>MNPAAEAEFNILLATDSYKVTHYKQYPPNTSKVYSYFECREKKTENSKLRKVKYEETVFYGLQYILNKYLKGKVVTKEKIQEAKDVYKEHFQDDVFNEKGWNYILEKYDGHLPIEIKAVPEGFVIPRGNVLFTVENTDPECYWLTNWIETILVQSWYPITVATNSREQKKILAKYLLETSGNLDGLEYKLHDFGYRGVSSQETAGIGASAHLVNFKVTDTVAGLALIKKYYGTKDPVPGYSVPAAEHSTITAWGKDHEKDAFEHIVTQFSSVPVSVVSDSYDIYNACEKIWGEDLRHLIVSRSTQAPLIIRPDSGNPLDTVLKVLEILGKKFPVTENSKGYKLLPPYLRVIQGDGVDINTLQEIVEGMKQKMWSIENIAFGSGGGLLQKLTRDLLNCSFKCSYVVTNGLGINVFKDPVADPNKRSKKGRLSLHRTPAG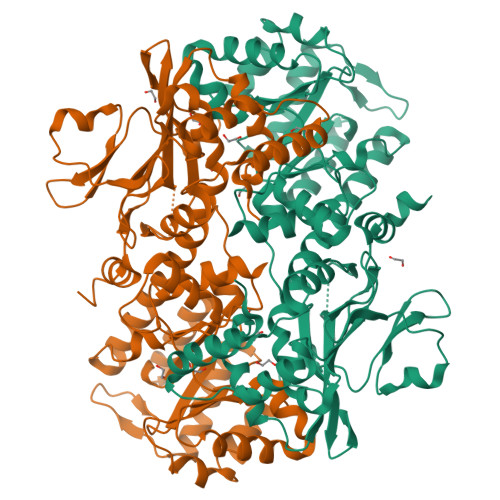NFVTLEEGKGDLEEYGQDLLHTVFKNGKVTKSYSFDEIRKNAQLNIELEAAHHLEHHHHHHHH[2x]> MSQSNRELVVDFLSYKLSQKGYSWSQPMAAVKQALREAGDEFELRYRRAFSDLTSQLHITPGTAYQSFEQVVNELFRDGVNWGRIVAFFSFGGALCVESVDKEMQVLVSRIASWMATYLNDHLEPWIQENGGWDTFVDLYG;> PIRYPWDVEC

The anti-apoptotic (pro-survival) proteins of the BCL-2 family include BCL-2, BCL-XL, MCL-1, BCL-w and BFL-1/A1. These proteins bind to and sequester the apoptosis effectors, as well as the apoptosis sensitizers, BIM, BID, PUMA, NOXA, BAD, BMF, HRK and BIK5,6. An elongated hydrophobic groove is thus formed along the surface of BCL-2 and BCL-XL proteins, spanning approximately 20 Å to serve as the binding site for the amphipathic α-helical BH3 domains of their pro-apoptotic partners. Herein we present cyclic peptides (CPs) with nanomolar-level binding affinities to BCL-2 or BCL-XL, and further reveal the structural and functional mechanisms of how these CPs target two proteins in a fashion that is remarkably different from traditional small-molecule inhibitors.

On the other hand, we obtained cp3 from the BCL-XL targeted screening. The affinities of cp3 to BCL-XL and BCL-2 were measured as 0.09 ± 0.01 μM and 0.24 ± 0.02 μM, showing a clearly improved binding to BCL-XL as compared with cp1. We surprisingly noticed that only the CPs containing a proline residue at the 6th position could be enriched in our screening against BCL-XL, implying this residue may be essential in the binding and selectivity of CPs. However, the buried interface between cp3 and BCL-XL is only 464.8 Å2, although its binding affinity to BCL-XL is the highest (0.09 ± 0.01 μM) among the three CPs. Subsequently, we further analyzed the interactions between cp3 and BCL-XL, and found that cp3, like a small protein, can be roughly divided into three sites that each directly contact the corresponding sites of BCL-XL respectively. These three sites of cp3 exhibit different properties, with Site 1’ (cp3-D8) negative charged, Site 2’ formed by linker of CPs (cADT) and Site 3’ composed by some hydrophobic residues (cp3-Y5, cp3-W7). The cp3-P6 forms a special molecular surface, which can perfectly fit into the unique interface formed by A104 of BCL-XL. Notably, the corresponding residue to BCL-XL A104 in BCL-2 is D111, which has a long side chain and would cause a steric clash with the surface of cp3 at P6. To test this hypothesis, we measured the binding affinity of BCL-2 D111A to cp3, and obtained a KD value of 0.09 ± 0.02 μM (comparable to the KD value of BCL-XL to cp3), indicating a nearly 3-fold improved affinity than that of BCL-2 WT (0.24 ± 0.02 μM).> QAQIT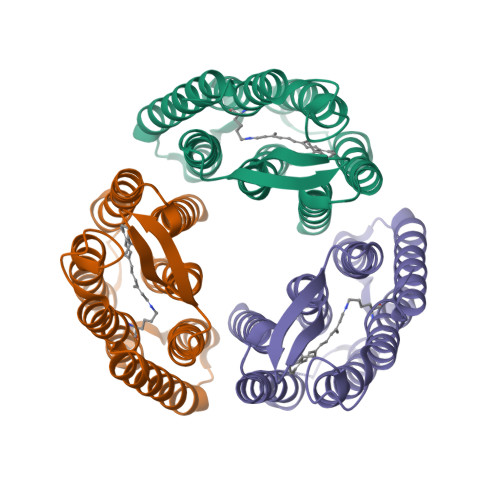GRPEWIWLALGTALMGLGTLYFLVKGMGVSDPDAKKFYAITTLVPAIAFTMYLSMLLGYGLTMVPFGGEQNPIYWARYADWLFTTPLLLLDLALLVDADQGTILALVGADGIMIGTGLVGALTKVYSYRFVWWAISTAAMLYILYVLFFGFTSKAESMRPEVASTFKVLRNVTVVLWSAYPVVWLIGSDGAGIVPLNIETLLFMVLDVSAKVGFGLILLRSRAIFGEAEAPEPSAGDGAAATSD>[2x]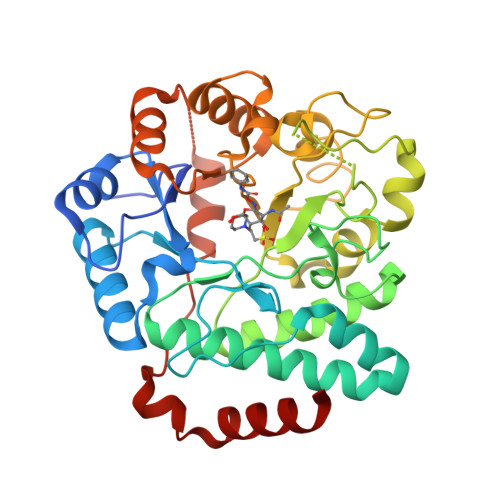MAHHHHHHMKTTPGPVMLDVVGTTLSRDDARRLAHPNTGGVILFARHFQNRAQLTALTDSIRAVREDILIAVDHEGGRVQRFRTDGFTVLPAMRRLGELWDRDVLLATKVATAVGYILAAELRACGIDMSFTPVLDLDYGHSKVIGDRAFHRDPRVVTLLAKSLNHGLSLAGMANCGKHFPGHGFAEADSHVALPTDDRTLDAILEQDVAPYDWLGLSLAAVIPAHVIYTQVDKRPAGFSRVWLQDILRGKLGFTGAIFSDDLSMEAAREGGTLTQAADAALAAGCDMVLVCNQPDAAEVVLNGLKARASAESVRRIKRMRARGKALKWDKLIAQPEYLQAQALLSSALA>[2x]GMKQPILNKLESLNQEEAISLHVPGHKNMTIGHLSQLSMTMDKTEIPGLDDLHHPEEVILKSMKQVEKHSDYDGYFLVNGTTSGILSVIQSFSQKKGDILMARNVHKSVLHALDISQQEGHFIETHQSPLTNHYNKVNLSRLNNDGHKLVVLTYPNYYGETF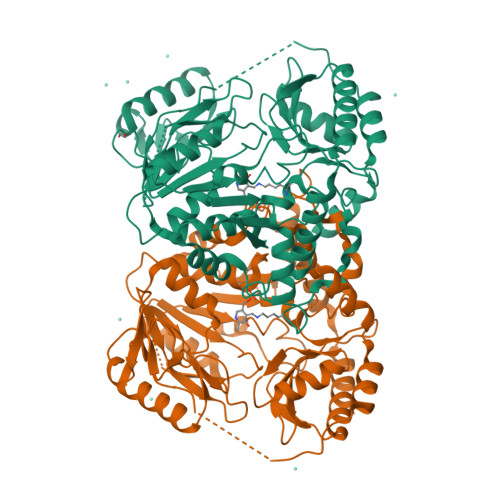NVEEVIKSLHQLNIPVLIDEAHGAHFGLQGFPDSTLNYQADYVVQSFHKTLPALTMGSVLYIHKNAPYRENIIEYLSYFQTSSPSYLIMASLESAAQFYKTYDSTLFFAKRAQLIECLENKGFEMLQVDDPLKLLIKYEGFTGHDIQNWFMNAHIYLELADDYQALAILPLWHHDDTYLFDSLLRKIEDMILPKKSVSKVKQTQLLTTEGNYKPKRFEYVTWCDLKKAKGKVLARHIVPYPPGIPIIFKGETITENMIELVNEYLETGMIVEGIKNNKILVEDE>[10x]DLDDVARIRLVLARELETINEYEAYA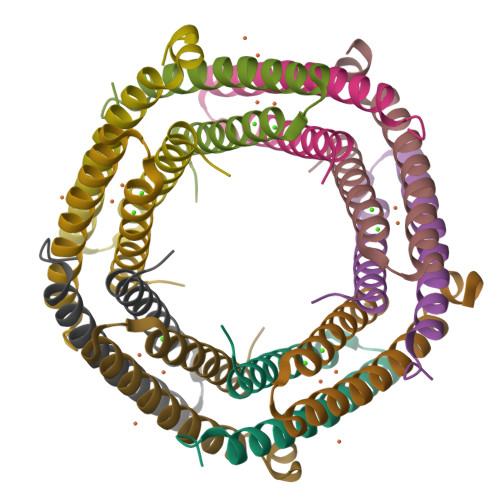RASSNPEVRAFFQHLAAEEKEHVSEAVHMLRMLDSGQNDHFA>MVSMKDFSGAELYTLEEYQYGKFEARMKMAAASGTVSSMFLYQNGSEIADGRPWVEVDIEVLGKSPGSFQSNIITGKAGAQKTSEKHHAVSPAADQAFHTYGLEWTPNYVRWTVDGQEVRKTEGGQVSNLTGTQGLRFNLWSSESAAWV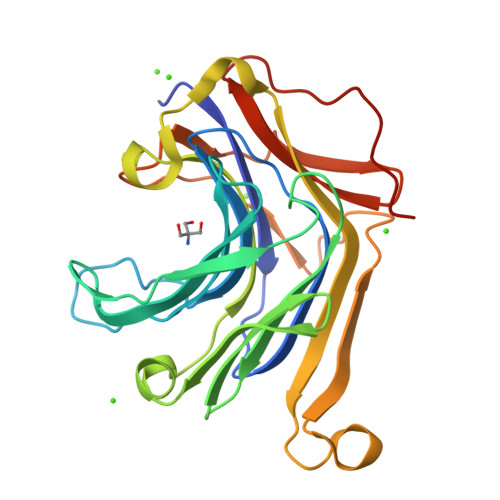GQFDESKLPLFQFINWVKVYKYTPGQGEGGSDFTLDWTDNFDTFDGSRWGKGDYTFDGNRVDLTDKNIYSRDGMLILALTRKGQESFNGQVPRDDEPAPL[2x]Here we analyze the mechanism of polyadenylation-independent Pol II termination mediated by the yeast Sen1 helicase. Cryo-electron microscopy structures of two pretermination intermediates show that Sen1 binds to Pol II and uses its adenosine triphosphatase activity to pull on exiting RNA in the 5′ direction. This is predicted to push Pol II forward, induce an unstable hypertranslocated state and destabilize the transcription bubble, thereby facilitating termination. Sen1 belongs to the ancient SF1b superfamily of helicases.

The Sen1-containing region of the map was improved using focused 3D classification and masked refinement, resulting in a local map at 3.3-Å resolution. The Sen1 structure features an ATPase domain with two ‘RecA lobes’ (lobes 1 and 2) and additional brace, stalk, β-barrel and prong modules. The structure of the pre-TC also shows that Sen1 binds the RNA transcript, burying up to 13 nt (register −35 to −23 relative to the Pol II active site) within its substrate-binding channel. Sen1 contacts RNA not only with its ATPase lobes 1 and 2 but also with its β-barrel, stalk and prong modules. The structure is consistent with prior work showing that a 30-nt nascent RNA is minimally required for Sen1-dependent termination.

> MNSNNPDNNNSNNINNNNKDKDIAPNSDVQLATVYTKAKSYIPQIEQVYQGTNPNIQEAKLLGELLQVLAEVPKGTHLFCDPILEPISIFSLTIFSFNEEATATWLKNHFNPILSVCDKCILNFARGKCKMLQHFAIQRHVPHEHVAKFNDIVCQWRVEAVFPILRNISVNDNTGINITNEIETAMYECLCNPHMLRLNKQLKATFEAIFKFFYDTKHRLLDVTNPLSIKTFISGVIFCWCEGSKEENEWSRAFLKDLYSRNFHINLSNLTPDIIEEVYIHILFLQNPANWTEIVVSQFWSRLLPVFNLFDKDVFIEYFQVPKNVESLKKTFKFPLEPIFKMWYNHLSKSYHDKPLDFLLRGLTMFLNKFGSEFWSKIEPFTFHSILDIIFNRDSFPIKLIKIQDNPIVEHQTEVYFQLTGSVTDLLSWTLPFYHALSPSKRIQMVRKVSMAFLRIIANYPSLKSIPKACLMNSATALLRAVLTIKENERAMLYKNDEFETVLLTKTDSRALLNNPLIQDIIIRSASNPNDFYPGLGAASASVATSTMMVLAECIDFDILLLCHRTFKLYSGKPISEIPISTNVLENVTNKIDLRSFHDGPLLAKQLLVSLKNINGLLIVPSNTAVAEAHNALNQKFLLLSTRLMEKFADILPGQLSKILADEDASQGFWSCIFSSDKHLYQAATNILYNTFDVEGRLEGILAILNSNLTVNLKNINVMLQRLINCEFYEPCPRAVRVLMDVVSAFVDPISGVFANFQTLKSQNTEKEFLKFWESCWLFLDTIYKFTLKWASKYDYSELENFTKDTLDLSRSLVDSFREFSDILHDQTKNLLLNVLETFKNMLYWLRLSDEVLLESCVRLIISTSDLAHEKHVKVDDSLVEMMAKYASKAKRFSNKLTEQQASEILQKAKIFNKALTEEVATEAENYRKEKELSRLGKVIDLTDSVPASPSLSPSLSSTIASSSAESRADYLQRKALSSSITGRPRVAQPKITSFGTFQSSANAKLHRTKPVKPLSKMELARMQLLNNRVVHPPSAPAFHTKSRGLSNKNDDSSSEESDNDIESARELFAIAKAKGKGIQTVDINGKVVKRQTAAELAKQELEHMRKRLNVDMNPLYEIILQWDYTRNSEYPDDEPIGNYSDVKDFFNSPADYQKVMKPLLLLESWQGLCSSRDREDYKPFSIIVGNRTAVSDFYDVYASVAKQVIQDCGISESDLIVMAYLPDFRPDKRLSSDDFKKAQHTCLAKVRTLKNTKGGNVDVTLRIHRNHSFSKFLTLRSEIYCVKVMQMTTIEREYSTLEGLEYYDLVGQILQAKPSPPVNVDAAEIETVKKSYKLNTSQAEAIVNSVSKEGFSLIQGPPGTGKTKTILGIIGYFLSTKNASSSNVIKVPLEKNSSNTEQLLKKQKILICAPSNAAVDEICLRLKSGVYDKQGHQFKPQLVRVGRSDVVNVAIKDLTLEELVDKRIGERNYEIRTDPELERKFNNAVTKRRELRGKLDSESGNPESPMSTEDISKLQLKIRELSKIINELGRDRDEMREKNSVNYRNRDLDRRNAQAHILAVSDIICSTLSGSAHDVLATMGIKFDTVIIDEACQCTELSSIIPLRYGGKRCIMVGDPNQLPPTVLSGAASNFKYNQSLFVRMEKNSSPYLLDVQYRMHPSISKFPSSEFYQGRLKDGPGMDILNKRPWHQLEPLAPYKFFDIISGRQEQNAKTMSYTNMEEIRVAIELVDYLFRKFDNKIDFTGKIGIISPYREQMQKMRKEFARYFGGMINKSIDFNTIDGFQGQEKEIILISCVRADDTKSSVGFLKDFRRMNVALTRAKTSIWVLGHQRSLAKSKLWRDLIEDAKDRSCLAYACSGFLDPRNNRAQSILRKFNVPVPSEQEDDYKLPMEYITQGPDEVKSNKDTKKRRVVDEGEEADKAVKKKKKEKKKEKKKSKADDKKKNNKKAESPSTSSGTKKKSSIFGGMSVPSAVVPKTFPDVDSNKKAAAVVGKKKNNKHVCFSDDVSFIPRNDEPEIKVTRSLSSVLKEKQLGLKETRTISPPEISNNEDDDDEDDYTPSISDSSLMKSEANGRNNRVASHNQNFSASIYDDPQVSQAKQTQVPAAITKHRSSNSVLSGGSSRILTASDYGEPNQNGQNGANRTLSQHVGNANQYSTAPVGTGELHETLPAHPQDSYPAEAEDPYDLNPHPQPQSSAFKGPGSGPTGTRNSSRRNASSSPFIPKKRKPRS>[4x]MREKGRRQAVRGPAFMFNDRGTSLTAEEERFLDAAEYGNIPVVRKMLEESKTLNVNCVDYMGQNALQLAVGNEHLEVTELLLKKENLARIGDALLLAISKGYVRIVEAILNHPGFAASKRLTLSPCEQELQDDDFYAYDEDGTRFSPDITPIILAAHCQKYEVVHMLLMKGARIERPHDYFCKCGDCMEKQRHDSFSHSRSRINAYKGLASPAYLSLSSEDPVLTALELSNELAKLANIEKEFKNDYRKLSMQCKDFVVGVLDLCRDSEEVEAILNGDLESAEPLEVHRHKASLSRVKLAIKYEVKKFVAHPNCQQQLLTIWYENLSGLREQTIAIKCLVVLVVALGLPFLAIGYWIAPCSRLGKILRSPFMKFVAHAASFIIFLGLLVFNASDRFEGITTLPNITVTDYPKQIFRVKTTQFTWTEMLIMVWVLGMMWSECKELWLEGPREYILQLWNVLDFGMLSIFIAAFTARFLAFLQATKAQQYVDSYVQESDLSEVTLPPEIQYFTYARDKWLPSDPQIISEGLYAIAVVLSFSRIAYILPANESFGPLQISLGRTVKDIFKFMVLFIMVFFAFMIGMFILYSYYLGAKVNAAFTTVEESFKTLFWSIFGLSEVTSVVLKYDHKFIENIGYVLYGIYNVTMVVVLLNMLIAMINSSYQEIEDDSDVEWKFARSKLWLSYFDDGKTLPPPFSLVPSPKSFVYFIMRIVNFPKCRRRRLQKDIEMGMGNSKSRLNLFTQSNSRVFESHSFNSILNQPTRYQQIMKRLIKRYVLKAQVDKENDEVNEGELKEIKQDISSLRYEL

A key component of SOCE has been identified as the TRPC channels, which are calcium-permeable, nonselective cation channels belonging to the TRP superfamily. Among the seven members in TRPC family, TRPC3, TRPC6, and TRPC7 are the closest homologues, and they are unique in being activated by the lipid secondary messenger diacylglycerol (DAG), a degradation product of the signaling lipid phosphatidylinositol 4,5-bisphosphate (PIP2). TPRC3, TRPC6, and TRPC7 share several functional domains, including N-terminal ankyrin repeats (AR), a transmembrane domain (TMD) with six transmembrane helixes (S1-S6), and a C-terminal coiled-coil domain (CTD). TRPC3 is abundantly expressed in the cerebellum, cerebrum, and smooth muscles, and it plays essential roles in the regulation of neurogenesis and extracellular/intracellular calcium signaling.

Here, we report the structure of full-length human TRPC3 (hTRPC3) in a lipid-occupied, inactive state at an atomic resolution of 3.3 Å using single-particle cryo-electron microscopy (cryo-EM). Detailed inspection of the TMD in TRPC3 reveals two unique features: a large elbow-like pre-S1 domain harboring a lipid-binding site (lipid 1), and an unusually long S3 helix forming an extracellular domain (ECD), along with the S1-S2 linker and S3-S4 linker. We identified two lipid-like densities, one sandwiched between the pre-S1 elbow and the S4-S5 linker, and the other wedged between the P loop and S6 of the adjacent subunit. The head group of lipid 1 is well defined in the density map, forming several hydrogen bonds and polar interactions with residues in the LD9, the pre-S1 elbow, half TM1, and the S4-S5 linker, while the two hydrocarbon tails are in contact with S1, S4, the pre-S1 elbow, and half TM1. We also identified a second lipid-like density (lipid 2) in the lateral fenestration of the pore domain, wedged between the P loop and S6 of adjacent subunit and forming both hydrophobic and hydrophilic interactions. Furthermore, a glycosylation site (N404) is observed in the S1-S2 loop, consistent with the prediction that TRPC3 is monoglycosylated in the extracellular side. The TRP helix forms an approximate right angle to the S6, in strong contrast to the TRPV1, TRPA1, and TRPM4 structures whose TRP helices form obtuse angles with S6. The pore adopts a closed conformation with the narrowest radius - at I658 and L654 on S6 close to the intracellular exit − of less than 1 Å, thus preventing ion passage. Presumably, the channel is trapped in a lipid-bound inactive state or the bound lipids are not the activator DAG. The selectivity filter is defined by the backbone carbonyl oxygens of I613, F614 and G615 located in the P loop.> DMPVERILEAELAVEPKTETYVEANMGLNPSSPNDPVTNICQAADKQLFTLVEWAKRIPHFSEL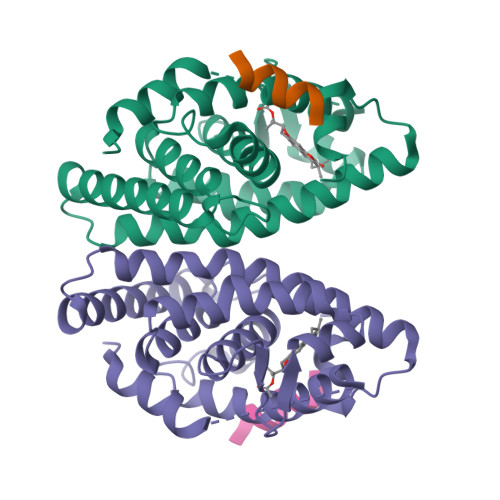PLDDQVILLRAGWNELLIASFSHRSIAVKDGILLATGLHVHRNSAHSAGVGAIFDRVLTELVSKMRDMQMDKTELGCLRAIVLFNPDSKGLSNPAEVEALREKVYASLEAYCKHKYPEQPGRFAKLLLRLPALRSIGLKCLEHLFFFKLIGDTPIDTFLMEMLEAP;> HKILHRLLQD> SMKKIDPLASTVVVRDGDLSSSFLAAARQCGRVTIDTETTGLSPKIDGLCTVQLHVPGVGTEIVRVDPTLQPTRLLQVLAAEEIVKGFHHAVFDLGFLRHTFQSKARSVVCSKVAAKILWPHDKDRQSLAGLAHLLLGVVLDKTPRLSDWSQPELTKTQVHYAAVDVEILPPILDELDR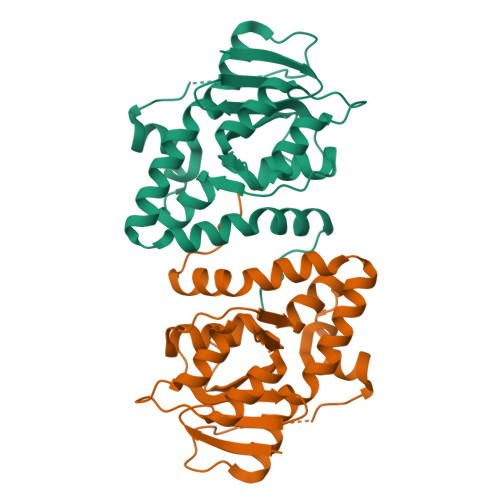LLSERQLRELAVACWHHIPAHVELLEHNLGDVFTY> MKAFTYERVNTPAEAALSAQRVPGAKFIAGGTNLLDLMKLEIETPTHLIDVNGLGLDKIEVTDAGGLRIGALVRNTDLAAHERVRRDYAVLSRALLAGASGQLRNQATTAGNLLQRTRCPYFYDTNQPCNKRLPGSGCAALEGFSRQHAVVGVSEACIATHPSDMAVAMRLLDAVVETITPEGKTR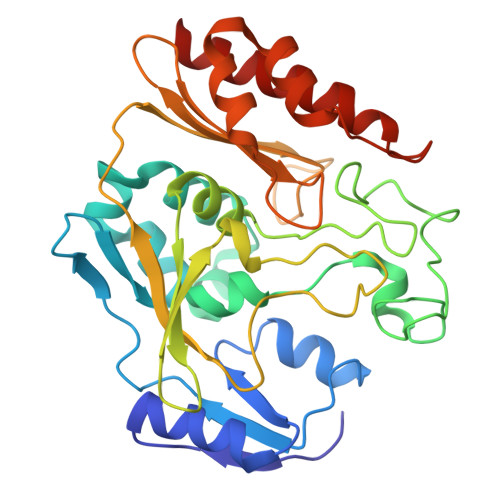SITLADFYHPPGKTPHIETALLPGELIVAVTLPPPLGGKHIYRKVRDRASYAFALVSVAAIIQPDGSGRVALGGVAHKPWRIEAADAQLSQGAQAVYDTLFASAHPTAENTFKLLLAKRTLASVLAEARAQA>MKQLLKLTGCVALAGLMSSCGSVQEEANYQIIPLPQEIVTSQVNPFILKSGVKILYPEGNEKMQRNAQFLADYLKTATGKDFSIEAGTEGKNAIVLALGSEVENPESYQLKVTDQGVTITAPTEAGVFYGIQTLRKSLPIALGADVALPAVEIKDAPRFGYRGAHFDVSRHFFTIDEVKTYIDMLALHNMNRLHWHITDDQGWRLEIKKYPKLTEIGSQRSGTVIGRNSGEYDNTPYGGFYTQEQAKEIVDYAAERYITVVPEIDLPGHMLAALAAYPELGCTGGPYEVWRQWGVADDVLCAGNDQVLKFLEDVYGELIEIFPSEYIHVGGDECPKVRWEKCPKCQARIKALGLKSDKNHSKEERLQSFVINHIEKFLNDHGRQIIGWDEILEGGLAPNATVMSWRGESGGIEAAKQKHDVIMTPNTYLYFDYYQAKDTENEPFGIGGYLPMERVYSYEPMPASLTPDEQQYIKGVQANLWTEYIATFSHAQYMVLPRWAALCEVQWSTPDKKNYEDFLSRLPRLIKWYDAEGYNYAKHVFDVKAEFTPNPADGTLDITLTTIDNAPIHYTLDGTEPTSTSPVYDGALKIKENADFSAIAIRPTGNSRVVSEKIDFSKSS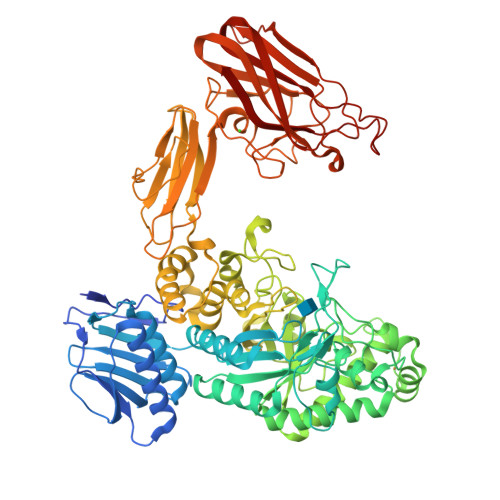MKPIVANQPVNKQYEFKGVSTLVDGLKGNGNYKTGRWIAFRGNDMDVTIDLKQPTEISSVAISTCVEKGDWVFDTRGLSVEVSEDGTNFTKVASEAYPAMKETDKNGVYDHKLTFTPVTAQYVKVIASPEKSIPEWHGGKSYPGFLFVDEITIN[3x]>MGMIGYFAEIDSEKINQLLESTEKPLMDNIHDTLSGLRRLDIDKRWDFLHFGLTGTSAFDPAKNDPLSRAVLGEHSLEDGIDGFLGLTWNQELAATIDRLESLDRNELRKQFSIKRLNEMEIYPGVTFSEELEGQLFASIMLDMEKLISAYRRMLRQGNHAL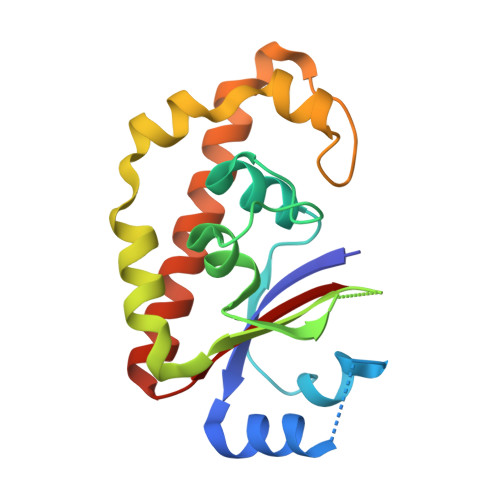TVIVG[2x]>GEADMDFLRNLFSQTLSLGSQKERLLDELTLEGVARYMQSERCRRVICLVGAGISTSAGIPDFRSPSTGLYDNLEKYHLPYPEAIFEISYFKKHPEPFFALAKELYPGQFKPTICHYFMRLLKDKGLLLRCYTQNIDTLERIAGLEQEDLVEAHGTFYTSHCVSASCRHEYPLSWMKEKIFSEVTPKCEDCQSLVKPDIVFFGESLPARFFSC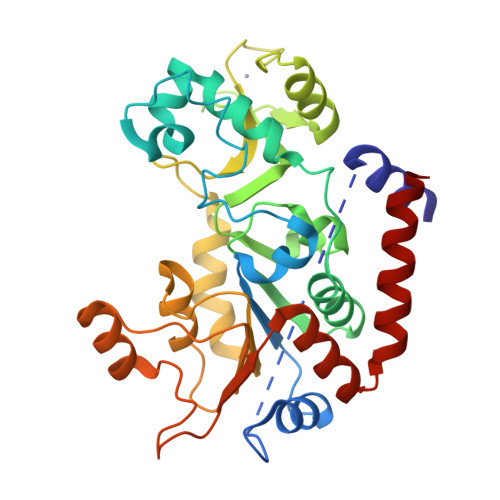MQSDFLKVDLLLVMGTSLQVQPFASLISKAPLSTPRLLINKEKAGQSDPFLGMIMGLGGGMDFDSKKAYRDVAWLGECDQGCLALAELLGWKKELEDLVRREHASIDAQS[3x]> SDRV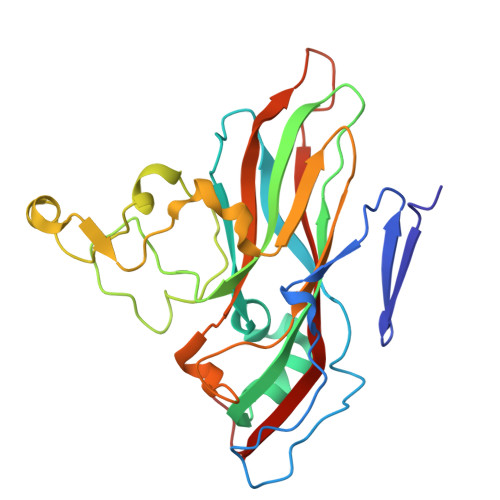SSDTAGNTATNTQSTVGRLFGFGQRHKGKHPASCADTATDKVLAAERYYTIKLASWTKTQESFDHIRVPLPHALAGENGGVFSSTLRRHYLCKCGWRIQVQCNASQFHAGSLLVFMAPEFDTSNHSTEVEPRADTAFKVDANWQKHAQILTGHAYVNTTTKVNVPLALNHQNFWQWTTYPHQILNLRTNTTCDLEVPYVNVCPTSSWTQHANWTLVIAVLTPLQYSQGSATTIEITASIQPVKPVFNGLRHTVV> CSALIKVLPGFENIFFAHSSWYTYAAMLRIYKHWDFNIVDKDTSSSRLSFSSYPGFLESLDDFYLLSSGLVLLQTTNSVYNKTLLQHVVPQSLLAWQRVRVASMMANNGKQWAEVFSKYNSGTYNNQYMVLDLKKVNLNHSLDEGTLYIVEQIPTYVEYSEQTAVLRRGYWPSYNIPFHEKVYNWSGYPILVKKLGLDYSYDLASRAKIFRRDQGKVTDMESMKYIMRYNNYKQDPYSKGDPCNTVCCREDLNSHSPSPGGCYDTKVADIYLASKYKAYA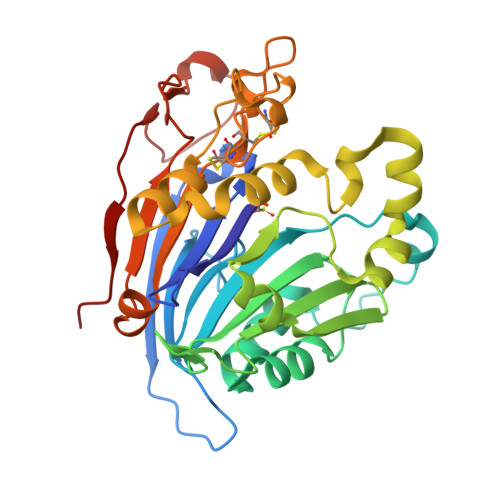ISGPTVQGGLPVFHWSRFNKTLHEGMPEAYNFDFITMKPIL> SMQELQGLDYCKPTRLDLLLDMPPVSYDVQLLHSWNNNDRSLNVFVKEDDKLIFHRHPVAQSTDAIRGKVGYTRGLHVWQITWAMRQRGTHAVVGVATADAPLHSVGYTTLVGNNHESWGWDLGRNRLYHDGKNQPSKTYPAFLEPDETFIVPDSFLVALDMDDGTLSFIVDGQYMGVAFRGLKGKKLYPVVSAVWGHCEIRMRYLN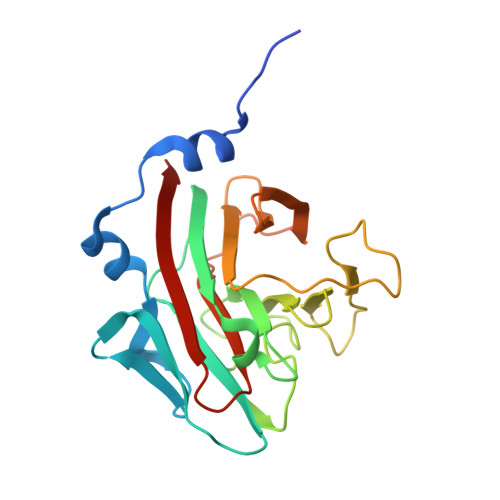GLDPE> MTDSVQTETTKGKIIINLFAPNLSGSTKEDDLIQKSLRDQLVESIRNSIAYPDTDKFAGLTRFIDEPGRNVFFVDGTRGAGKTTFINSVVKSLNSDQDDVKVNIKCLPTIDPTKLPRHEPILVTVTARLNKMVSDKLKGYWASNDYRKQKEQWQNHLAQLQRGLHLLTDKEYKPEYFSDALKLDAQLDYSIGGQDLSEIFEELVKRACEILDCKAILITFDDIDTQFDAGWDVLESIRKFFNSRKLVVVATGDLRLYSQLIRGKQYENYSKTLLEQEKESVRLAERGYMVEHLEQQYLLKLFPVQKRIQLKTMLQLVGEKGKAGKEEIKVKTEPSMQDIDAIDVRQAIGDAVREGLNLREGSDADMYVNELLKQPVRLLMQVLQDFYTKKYHATSVKLDGKQSRNERPDELSVPNLLRNALYGSMLSNIYRAGLNYEQHRFGMDSLCKDIFTYVKQDRDFNTGFYLRPQSESEALRNCSIYLASQVSENCQGSLSKFLQMLLVGCGSVSIFNQFVTE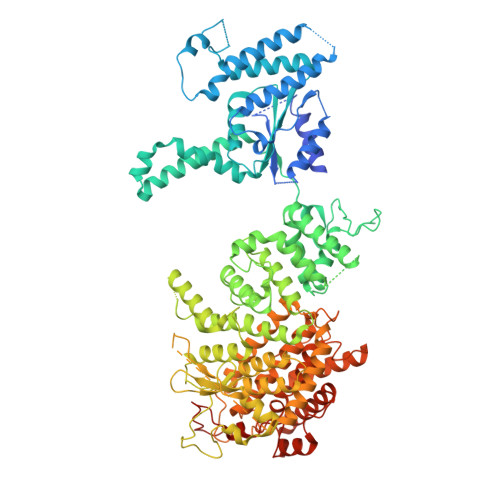LARAENDREKFEQLISEYVAYMSVGRIESASHWANRCCAVVANSPNDEKIGVFLGMVQLNRKSRQNMPEGYKKFNIDTENGLAKAAMASSLSTVASNNLMDFCSVFNLIGAIADISACRCERSAITNAFNKVIAQTTCIVPPWSEAAVRAEMKGSSKSADNDAAVLDVDLDPKDDGVIDESQQDDATEFSDAITKVEQWLKNVNEIEIGIRPSALLIGKVWSRFYFNLNNVADQHKTRLYRNAEHGRMASQSNAAKIMRFNVLAFLHAVLVEESLYHSVSDREYIGEGLRLNPVTSVDEFEKKIKIIGEKLKADNKTWKNTHPLFFLLISCPILHPFIFPIGGINCSVKALNKETSFNKLIDEIVGDKLLSDEEWDYLTKNNDQKTNTRQQIFQNTITSLNSSTIVGASYDKDTPARKTKSPSLGDSEEK5-[[3-(trifluoromethyl)phenyl]methyl]-1,4,6,7-tetrahydroimidazo[4,5-c]pyridine 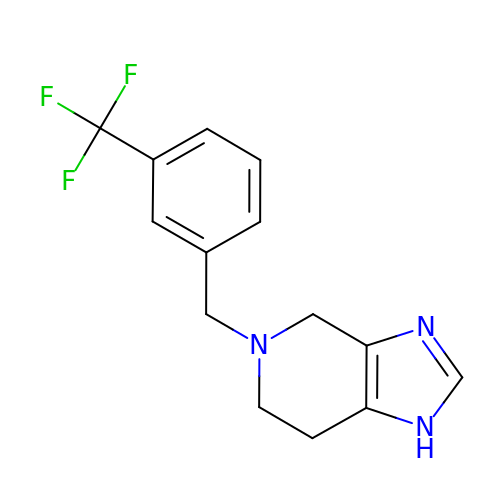| C14 H14 F3 N3 | FOPKRYDZNCKFAQ-UHFFFAOYSA-N> MSFREQDIYL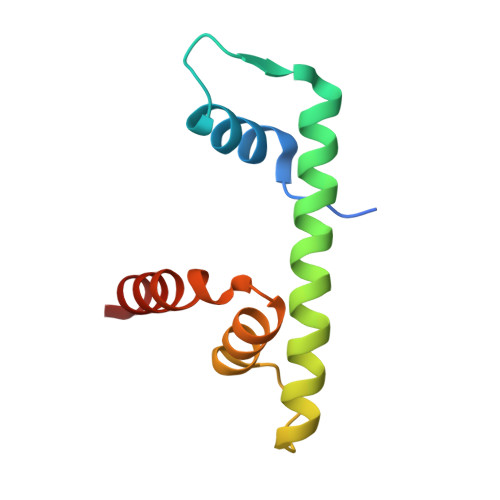PIANVARIMKNAIPQTGKIAKDAKECVQECVSEFISFITSEASERCHQEKRKTINGEDILFAMSTLGFDSYVEPLKLYLQKFRE> MQNITAMPRTIWTGLLLGLLLAGCRGMISSKPPVHPNLNMDFQEKF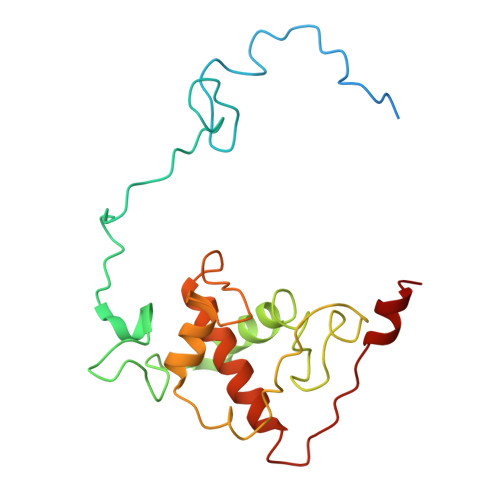EAQELNPFFADRRAMRPPVPGTVPRGLLKEDTPFYFGKTADGAYVERIPVAVTPELVARGRERYNIYCAVCHGQAGDGQGIIMRGNYGYTPAPSFHDDRLRNVEDGYIFDVISHGVRNMPAYGHQIPVADRWAIVAYVRALQRSQHATAADVPEEVRARLQGE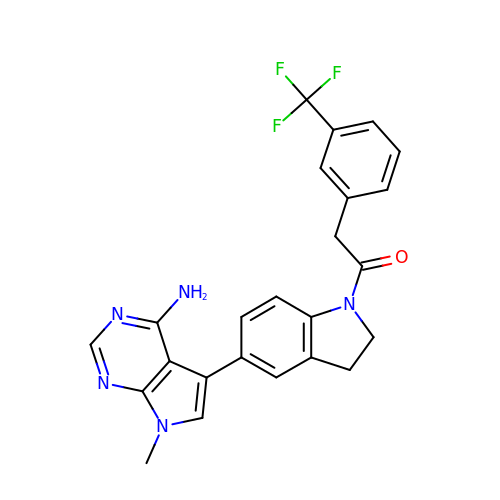1-[5-(4-amino-7-methyl-7H-pyrrolo[2,3-d]pyrimidin-5-yl)-2,3-dihydro-1H-indol-1-yl]-2-[3-(trifluoromethyl)phenyl]ethanone | C24 H20 F3 N5 O | SIXVRXARNAVBTC-UHFFFAOYSA-N In 2020, Tan et al. discovered that BktB from Cupriavidus necator is a polyketoacyl-CoA thiolase and demonstrated its activity to produce polyketides, including TAL, through repetitive non-decarboxylative Claisen condensations with acetyl-CoA as both precursor and extension unit in vitro and in vivo in E. coli. One candidate, BktBbr from Burkholderia sp. RF2-non_BP3, exhibits approximately 30-fold higher activity in vitro and supports 30-fold higher TAL titers in Escherichia coli compared to the original enzyme. Additionally, we resolve the high-resolution X-ray structure of BktBbr with three different substrates: acetyl-CoA, acetoacetyl-CoA, and butyryl-CoA.

BktBbr has a special loop region that stabilizes the tetrameric structure. Deleting this loop region eliminated >95% TAL production. Comparing the apo structure with the structures covalently bound by CoA esters, no obvious structural changes were observed. High-resolution X-ray structures of the apo enzyme and enzyme bound to various CoA substrates allowed us to perform rational mutagenesis and generate mutants that were more productive when expressed in E. coli. The tunnel architecture in BktBbr appears optimized to facilitate substrate positioning and product release, which may underlie its superior kcat and in vivo product titer compared to BktBcn.

>GHMSNAAKEVVVVSGVRTAIGDFGGSLKDFSPTDLGAKVVSEVLSRANVSGDAVGHVVFGHVVNTEPKDMYLARVAAINGGVAQHTPALTVNRLCGSGLQAIVSAAQTIMLGDADVAIGGGSENMSRAPYTVPSARFGQRMGDAKLVDMMLGALHDPFQTIHMGVTAENVARKYGITRDAQDALALESHRRAARAIAEGRFKDQILPISIRTKKGEVAFDTDEHVRHDAGPDDFTKLKPVFVKEDGTVTAGNASGINDAAAAVLMMSADAARAQGVKPLARLVAYAHAGVDPAYMGIGPVPATQKALERAGLKITDLDVIEANEAFAAQACAVTQELGLDPAKVNPNGSGISLGHPIGATGALITVKALYELKRIGGRYALVTMCIGGGQGIAAIFENI[2x]>[4x]MRGSHHHHHHGSLSSSPSEILQELGKGSTHPQPGVSPPAAPAAPGPKDGPGETDAFGNSEGKELVASGENKIKQGLLPSLEDLLFYTIAEGQEKIPVHKFITALKSTGLRTSDPRLKECMDMLRLTLQTTSDGVMLDKDLFKKCVQSNIVLLTQAFRRKFVIPDFMSFTSHIDELYESAKKQ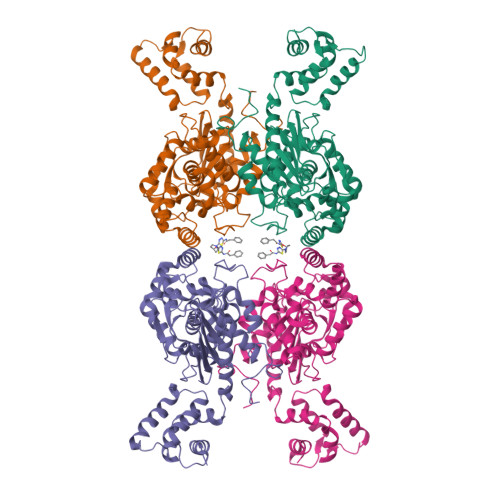SGGKVADYIPQLAKFSPDLWGVSVCTADGQRHSTGDTKVPFCLQSCVKPLKYAIAVNDLGTEYVHRYVGKEPSGLRFNKLFLNEDDKPHNPMVNAGAIVVTSLIKQGVNNAEKFDYVMQFLNKMAGNEYVGFSNATFQSERESGDRNFAIGYYLKEKKCFPEGTDMVGILDFYFQLCSIEVTCESASVMAATLANGGFCPITGERVLSPEAVRNTLSLMHSCGMYDFSGQFAFHVGLPAKSGVAGGILLVVPNVMGMMCWSPPLDKMGNSVKGIHFCHDLVSLCNFHNYDNLRHFAKKLDPRREGGDQRHSFGPLDYESLQQELALKETVWKKVSPESNEDISTTVVYRMESLGEKS>[3x]GAQKKTQKTYIPWSNGKLVVSEEGRYLKHENGTPFFWLGETGWL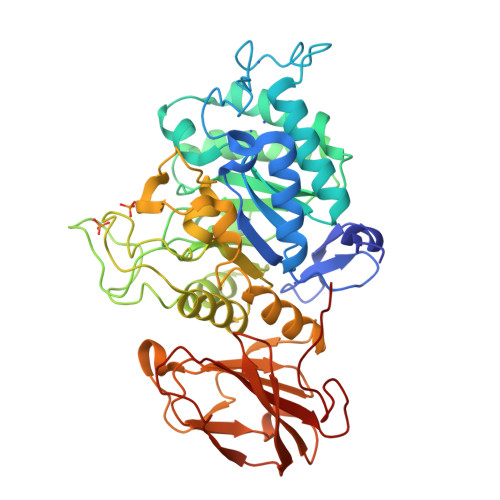LPERLNRDEAEYYLEQCKRRGYNVIQVQTLNNVPSMNIYGQYSMTDGYNFKNINQKGVYGYWDHMDYIIRTAAKKGLYIGMVCIWGSPVSHGEMNVDQAKAYGKFLAERYKDEPNIIWFIGGDIRGDVKTAEWEALATSIKAIDKNHLMTFHPRGRTTSATWFNNAPWLDFNMFQSGHRRYGQRFGDGDYPIEENTEEDNWRFVERSMAMKPMKPVIDGEPIYEEIPHGLHDENELLWKDYDVRRYAYWSVFAGSFGHTYGHNSIMQFIKPGVGGAYGAKKPWYDALNDPGYNQMKYLKNLMLTFPFFERVPDQSVIAGQNGERYDRAIATRGNDYLMVYNYTGRPMEVDFSKISGAKKNAWWYTTKDGKLEYIGEFDNGVHKFQHDSGYSSGNDHVLIVVDSSKDYVKKDCYQIDTHE Here, we report on the structure and reactivity of such a deviant enzyme, termed CooS‐VCh. Its structure reveals the typical CODH scaffold, but contains an iron‐sulfur‐oxo hybrid‐cluster. Although closely related to true CODHs, CooS‐VCh catalyzes neither CO oxidation, nor CO2 reduction. The active site of CooS‐VCh undergoes a redox‐dependent restructuring between a reduced [4Fe‐3S]‐cluster and an oxidized [4Fe‐2S‐S*‐2O‐2(H2O)]‐cluster.

Two molecules were identified in the asymmetric unit and the structure was rebuilt and refined using reflections extending to 1.35 Å resolution. Two μ2‐bridging ligands between Fe2–Fe4 and Fe3–Fe4 were modeled as oxygen and not sulfur, based on the lack of anomalous scattering contribution, shorter Fe−O bond lengths and less electron density at this position. The mixed cluster can be divided into two subsites: a [2Fe‐2S‐H2O] site and a [2Fe‐S‐2O‐H2O] site, together generating two almost perpendicular planes fused along one side (106° plane angle between Fe1‐S1‐Fe2‐S2 and Fe2‐S2‐Fe3‐Fe4). The Fe1 and Fe2 atoms of the [2Fe‐2S] subsite are coordinated by Cys338 and Cys480, respectively, with Asn337 in short hydrogen‐bonding distance to the water at the [2Fe‐2S] subsite (2.4 Å). Fe4 is coordinated by three oxygens and one sulfur: the bridging oxo/hydroxo ligands, O1 (1.64 Å) and O2 (1.98 Å), a hydroxo/water ligand (2.07 Å) and S3* (2.42 Å) that is part of a persulfide formed with the thiolate Sγ of Cys521. Fe3 is coordinated by two oxygen and two sulfur ligands, O2 in the μ2‐oxo‐bridge (1.86 Å), Oϵ1 from Glu295 (2.23 Å), the thiolate of Cys449 (2.36 Å) and S2 (2.32 Å). All iron atoms in the oxidized cluster are tetrahedrally coordinated. In the oxidized state, two channels with widest diameter of approx. 4 Å converge near the hybrid‐cluster. However, there is no access to the hybrid‐cluster in the oxidized state, because the S3 atom, now part of a persulfide, blocks the path to the cluster (closed conformation in Figure 7A).

>MATKTSIHPSVNELYQRLAEDQLSNCFDRFDPQEKIRCNYCELGVSCQLCSNGPCRINEKVGATLGVCGINADGMAMRYMLLRNVMGTSTYTYHAYEAYKTLKMTALGNTPFTITDKDKLYQMAKDLELNTEGKPEDVAVRLSDFLIWELYRDYDEPGKMIEVYAPLKRKEVWRKLGIYPAGPLHELKDAAASCLTNVDGDYVSLATKGLRLGLSCIYGAQIGLELVQDILFGTGMPHEMDVDLGIFDADYINIVFNGHEPFVGVALILAAKEAVNQDKAKAAGAKSLRIYGSIESGQEVVQRFQKDEVFRGLTGNWLTIEPMLATGAVDVLAMDMNCSPPNLGPLAEKYGATLVSVSRLVRFPGIHHFLDYKPSEVREIAQKIIDIAVDSFKNKRHGKITPKIPANIQKAITGFTPEAILKALGGSINPLIEVIKAGKIKGAVGLINCTTLKNGPQDYVTVNLAKELIKRDILILSGGCGNHALEVAGLCNLDAINLAGPGLSEVCRNLNIPPVLSFGTCTDTGRISLVVTALANALNVDTADLPVAVTAPMYMEQKATIDALFALAYGLYTHVAPDPPVMGAPNLVKLLTRDLPSITGGRIAVGSDPVKVADDILAHINDRRAKLGI[2x]>MNITGKGAYDTGTYANLFQRSGYREDEIKARLEQTWNDLFYGDEHTRIYYPVGDDKGYMLDTGNDDVRSEGMSYGMMMAVQMDKKHEFDRLWNYAYTYMQHTEGRYKDYFAWHCKPDGTRLSPGPAPDGEEFFAMALFFASNRWGDGPAPYDYQAQARKILHACLHQGEQGEGDPMWEPSNRLIKFIPELPFSDPSYHLPHFYELFAQYANEQDRTFWKEAAEASRAYLRTACHPVTGLSPEYANYDGTPAPVQLHGDFRHFYSDAYRVAANVALDWEWFRKDPWQVQQSNRIQAFFSDIDVSDYRRYTIEGEPFNEPAASPVGLLATNAMASLAADGPDADSFVKRFWNTPLRQGKRRYYDNCLYFFTMLALSGNYRVY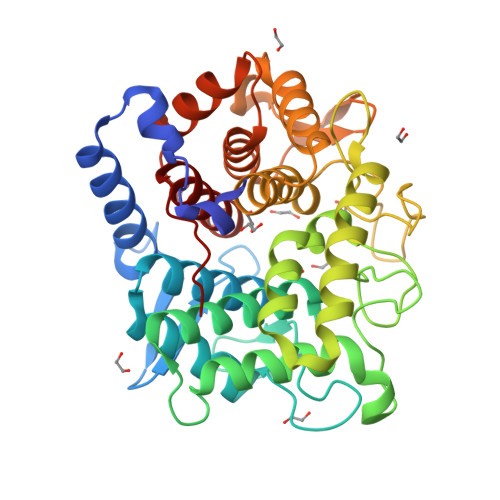QQ[2x]> GSHMMFLVVGQGNPGERYARTRHNLGFMVLDRLGLSFRPRGEALVAEAEGGLFLKPLTYYNLTGRAVAPLARFYKIPPERILVVHDEMDLPLGRIRFKAGGSAAGNRGVLSIEEALGTRAFHRLRLGIGKPPDPSRGAEYVLSPFREEELPVVERVLEAAKEAVWCWVREG

Peptidyl-tRNA hydrolase (Pth) hydrolyzes the ester bond between the peptide and the tRNA of peptidyl-tRNA molecules, which are the products of aborted translation, to prevent cell death by recycling tRNA. Pth releases the tRNA from the peptidyl-tRNA, by cleaving the ester bond between the C-terminal end of the peptide and the 2′- or 3′-hydroxyl group of the adenosine at the 3′-end of the tRNA (A76), and makes the free tRNA available for further rounds of protein synthesis. Pth1 adopts an α/β globular structure and functions as a monomeric enzyme, while Pth2 has a structure similar to thioredoxin and acts as a homodimeric enzyme. Here, we present the crystal structure of Thermus thermophilus Pth (TtPth) in complex with adenosine 5′-monophosphate (AMP), a mimic of A76.

Thus, we next used a C-terminal α-helix (C-terminal 16 amino acid residues) deletion mutant and performed crystallization trials. Instead, we obtained crystals of TtPth in which the C-terminal three amino acid residues (Arg165-Glu166-Gly167) of a crystallographically-related neighboring TtPth molecule penetrate and interact with the active site cleft (A−C and S2B). Hereafter, we refer to this structure as TtPth⋅tripeptide. The TtPth⋅tripeptide structure showed that the tripeptide, Arg165-Glu166-Gly167, interacts with 7 amino acid residues in the active site cleft (Asn9, Tyr14, His19, Try55, Tyr56, Asn57, and Leu138). In addition, the main chain carbonyl oxygen of Arg165 forms a hydrogen bond with the main chain amide nitrogen of Asn57. Furthermore, the main chain carbonyl oxygen of Glu166 forms a hydrogen bond with the side chain amide nitrogen of Asn9. In addition, one of the C-terminal carboxyl oxygens of Gly167 forms a hydrogen bond with the side chain amide nitrogen of Asn57. In terms of the crucial regions for the substrate binding, the Cα atom distances of the closest residues between the gate loop (Ala100) and the base loop (Asp85) in TtPth⋅tripeptide and apo TtPth are 9.26 Å and 7.69 Å, respectively. The cleft between the base loop and the gate loop seems to open upon peptide binding. The crystal structure of TtPth⋅tripeptide showed that the C-terminal amino acid residues of a crystallographically-related neighboring molecule bind to the active site cleft, in a manner mimicking a peptide moiety of the substrate.>[2x]MIRLYPEQLRAQLNEGLRAAYLLLGNDPLLLQESQDAVRQVAAAQGFEEHHTFSIDPNTDWNAIFSLCQAMSLFASRQTLLLLLPENGPNAAINEQLLTLTGLLHDDLLLIVRGNKLSKAQENAAWFTALANRSVQVTCQTPEQAQLPRWVAARAKQLNLELDDAANQVLCYCYEGNLLALAQALERLSLLWPDGKLTLPRVEQAVNDAAHFTPFHWVDALLM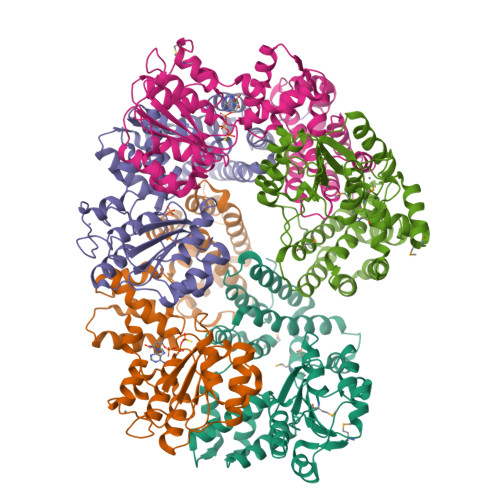GKSKRALHILQQLRLEGSEPVILLRTLQRELLLLVNLKRQSAHTPLRALFDKHRVWQNRRGMMGEALNRLSQTQLRQAVQLLTRTELTLKQDYGQSVWAELEGLSLLLCHKPLADVFIDG;>MSYQVLARKWRPQTFADVVGQEHVLTALANGLSLGRIHHAYLFSGTRGVGKTSIARLLAKGLNCETGITATPCGVCDNCREIEQGRFVDLIEIDAASRTKVEDTRDLLDNVQYAPARGRFKVYLIDEVHMLSRHSFNALLKTLEEPPEHVKFLLATTDPQKLPVTILSRCLQFHLKALDVEQIRHQLEHILNEEHIAHEPRALQLLARAAEGSLRDALSLTDQAIASGDGQVSTQAVSAMLGTLDDDQALSLVEAMVEANGERVMALINEAAARGIEWEALLVEMLGLLHRIAMVQLSPAALGNDMAAIELRMRELARTIPPTDIQLYYQTLLIGRKELPYAPDRRMGVEMTLLRALAFHPRMPLPEPEVPRQ[6x];>MRWYPWLRPDFEKLVASYQAGRGHHALLIQALPGMGDDALIYALSRYLLCQQPQGHKSCGHCRGCQLMQAGTHPDYYTLAPEKGKNTLGVDAVREVTEKLNEHARLGGAKVVWVTDAALLTDAAANALLKTLEEPPAETWFFLATREPERLLATLRSRCRLHYLAPPPEQYAVTWLSREVTMSQDALLAALRLSAGSPGAALALFQGDNWQARETLCQALAYSVPSGDWYSLLAALNHEQAPARLHWLATLLMDALKRHHGAAQVTNVDVPGLVAELANHLSPSRLQAILGDVCHIREQLMSVTGINRELLITDLLLRIEHYLQPGVVLPVPHL[2x]>CCCCCIIIII[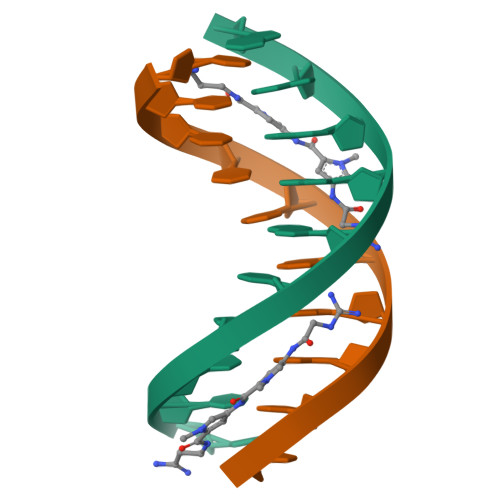4x]>[2x]HHHHHHSSGLVPRGSHQSQAPIPKDIAYHTLTKALLFPDIDQYQHWHHVAPMLAKMLVDGKYSIHQQYEYLCLFAQLVAPVLGPYPSPGRDVYRCTLGGNMTVELSQNFQRSGSTTRIAFEPVRYQASVGHDRFNRTSVNAFFSQLQLLVKSVNIELHHLLSEHLTLTAKDERNLNEEQLTKYLTNFQVKTQYVVALDLRKTGIVAKEYFFP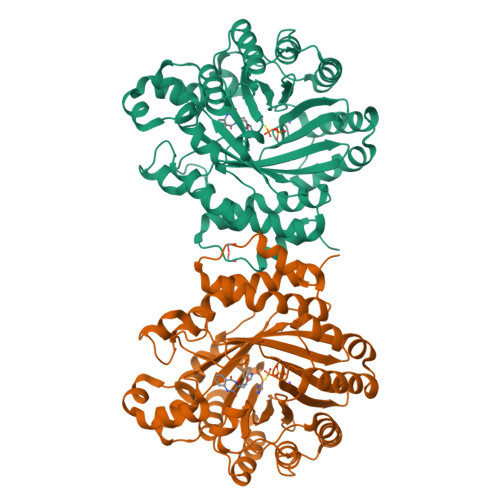GIKCAATGQTGSNACFGAIRAVDKDGHLDSLCQLIEAHFQQSKIDDAFLCCDLVDPAHTRFKVYIADPLVTLARAEEHWTLGGRLTDEDAAVGLEIIRGLWSELGIIQGPLEPSAMMEKGLLPIMLNYEMKAGQRLPKPKLYMPLTGIPETKIARIMTAFFQRHDMPEQAEVFMENLQAYYEGKNLEEATRYQAWLSFAYTKEKGPYLSIYYFWPE>MSKIKMKVPLVEMDGDEMTRIIWRLIKENLLEPYIELNTEYYDLGLENRDKTEDQVTIDAARAIQKYGVGVKCATITPNAQRVEEYNLKKMWKSPNGTIRAILDGTVFRAPIVVNSIKPFVKGWKKPISIARHAYGDVYKNVEYYVPSAGKAELVFTSENGEVSRQTIHEFDGPGVIMGMHNTDKSIRSFARACFNYALDMNQDLWFSTKDTISKTYDHRFKDIFQEIYENEYKEKFEAKNLQYFYTLIDDAVARIIRSEGGMVWACKNYDGDVMSDMVASAFGSLAMMTSVLVSPDGKYEFEAAHGTVTRHYYKHLKGEETSTNSMATIFAWTGALKKRG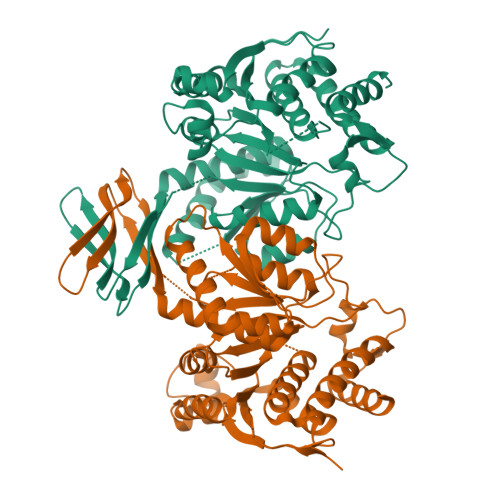ELDGIKELVDFATKLEQASVQTIENGVMTKDLASLSEVPEKKIVNTEDFLKEIRKTFEGMA[4x]> MTDHYKAVEALISDQAVDSFETSPNPRFKQIMQSLVRHLHDFVSEVELTEQEWFEGIRFLTATGQKCDGKVRQEFILLSDTLGVSMLVDAINHRQSTNATETTVFGPFFIEGMPDRGYGENMALTDGVPALVYGRVLDVQGRPVVGAVLDVWQTADNGMYSGQDPDQPFGNLRGRYRSDNDGCFAIQTTVPVCYPIPTDGPVGEMLDAANRHAWRPAHLHFMIQ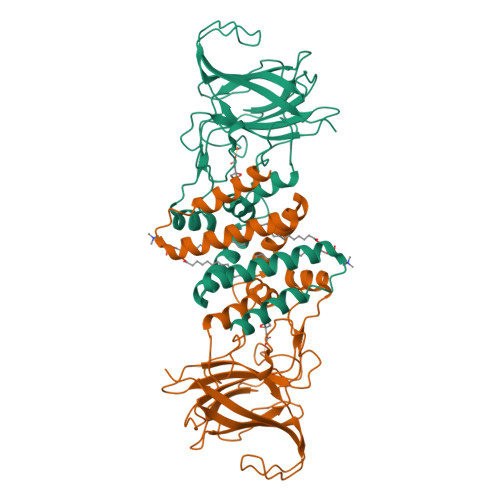APGYRKLVTHLFNSDDPYLDSDAVFGVKGSLQVKYEDRPAHDEDAGGLDMPYPYKSAYYEFVMEAE>ACAMLERAKVKDEWAKAYGIGAARSKFGDALWRNVFNYAPNARDIFESVNSKDMASPEFKAHIARVLGGLDRVISMLDNQATLDADLAHLKSQHDPRTIDPVNFVVFRKALIATVAGTFGVCFDVPAWQGCYNIIAKGITGSDAA[6x];>[6x]DYVCGPLQRLKVKRQWAEAYGSGNSREEFGHFIWSHVFQHSPAARDMFKRVRGDNIHTPAFRAHATRVLGGLDMCIALLDDEPVLNTQLAHLAKQHET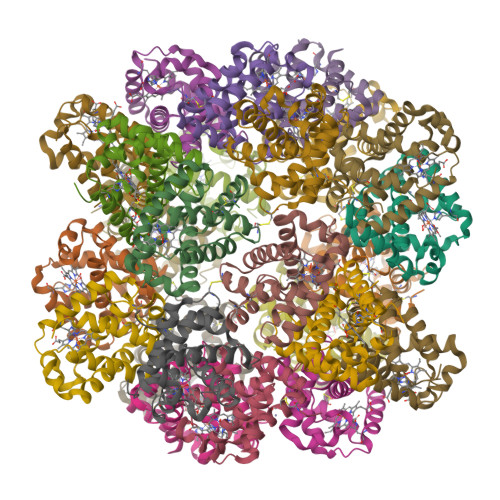RGVEAAHYDTVNHAVMMGVENVIGSEVFDQDAWKPCLNVITNGIQG;>[6x]AANCADAAAAIVQAQWEDVWSAAAAAASRVSAGEEVFAALFKMVPAAKNLFTRVNVADINSPEFQGHVVRVMGGLDILINALDDIPTLESMLDHLAGQHAVRDGVTGAGFQLMATVLMESLPQVVEGFNPDAWASCLAGIAAAISSAL;>AASCTTEDRREMQLMWGNVWSAQFTGRRIAIAQAVFKDLFANVPDAVGLFGAVKGDEVNSNEFKAHCIRVVNGLDSSIGLLSDPATLNEQLSHLATQHKARSGVTKGGFSAIAQSFLRVMPQVASCFNPDAWSRCFNRITTGMTEPLPA[6x]> GCCCGGAUAGCUCAGUCGGUAGAGCAGCGGAGCUGUUAGUCUACGUGGACCGACAAAGA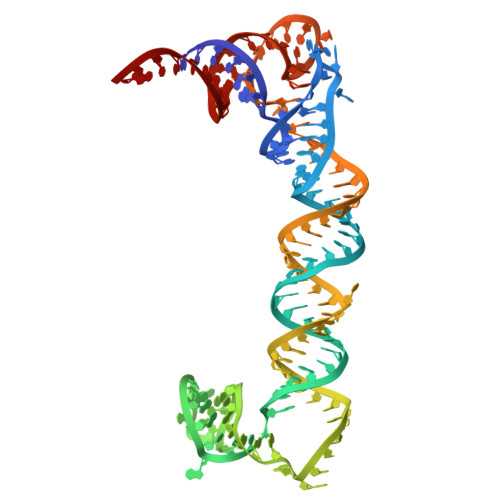CAGAUUCUUUGAGGGAGCUAAGCUCAACGUAGUUCUAACAGCUCCGCGGGUCCAGGGUUCAAGUCCCUGUUCGGGCGCCA>[2x]MVGRNSAIAAGVCGALFIGYCIYFDRKRRSDPNFKNRLRERRKKQKLAKERAGLSKLPDLKDAEAVQKFFLEEIQLGEELLAQGEYEKGVDHLTNAIAVCGQPQ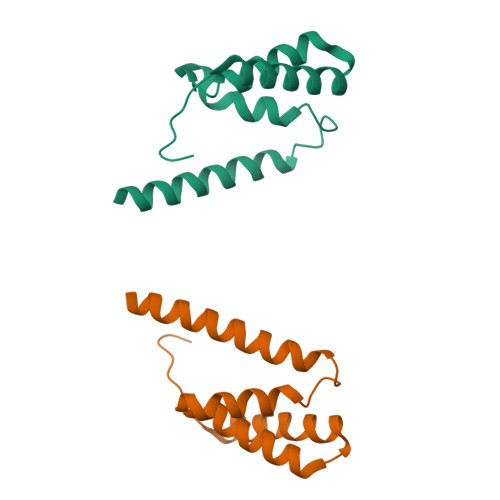QLLQVLQQTLPPPVFQMLLTKLPTISQRIVSAQSLAEDDVE> MSLSFCGNNISSYNIYHGVLQNPCFVDALNLVPHVFLLFITFPILFIGWGSQSSKVQIHHNTWLHFPGHNLRWILTFALLFVHVCEIAEGIVSDSQRASRHLHLFMPAVMGFVATTTSIVYYHNIETSNFPKLLLALFLYWVMAFITKTIKLVKYWQLGWGMSDLRFCITGVMVILNGLLMAVEINVIRVRRYVFFMNPQKVKPPEDLQDLGVRFLQPFVNLLSKATYWWMNTLIISAHRKPIDLKAIGKLPIAMRAVTNYVCLKEAYEEQKKKAADHPNRTPSIWLAMYRAFGRPILLSSTFRYLADLLGFAGPLCISGIVQRVNEPKNNTTRFSETLSSKEFLENAHVLAVLLFLALILQRTFLQASYYVTIETGINLRGALLAMIYNKILRLSTSNLSMGEMTLGQINNLVAIETNQLMWFLFLCPNLWAMPVQIIMGVILLYNLLGSSALVGAAVIVLLAPIQYFIATKLAEAQKSTLDYSTERLKKTNEILKGIKLLKLYAWEHIFCKSVEETRMKELSSLKTFALYTSLSIFMNAAIPIAAVLATFVTHAYASGNNLKPAEAFASLSLFHILVTPLFLLSTVVRFAVKAIISVQKLNEFLLSDEIGEDSWRTGEGTLPFESCKKHTGVQSKPINRKQPGRYHLDNYEQARRLRPAETEDVAIKVTNGYFSWGSGLATLSNIDIRIPTGQLTMIVGQVGCGKSSLLLAILGEMQTLEGKVYWNNVNESEPSFEATRSRSRYSVAYAAQKPWLLNATVEENITFGSSFNRQR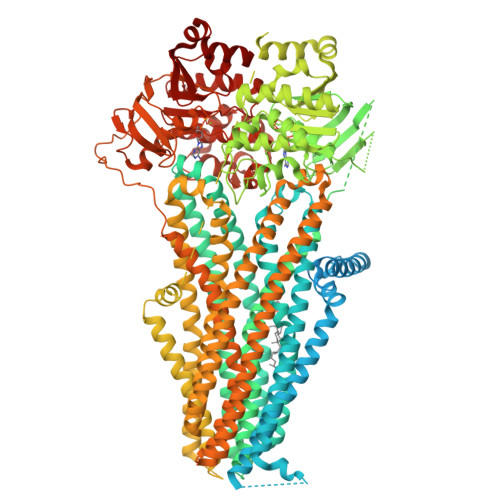YKAVTDACSLQPDIDLLPFGDQTEIGERGINLSGGQRQRICVARALYQNTNIVFLDDPFSALDIHLSDHLMQEGILKFLQDDKRTVVLVTHKLQYLTHADWIIAMKDGSVLREGTLKDIQTKDVELYEHWKTLMNRQDQELEKDMEADQTTLERKTLRRAMYSREAKAQMEDEDEEEEEEEDEDDNMSTVMRLRTKMPWKTCWWYLTSGGFFLLFLMIFSKLLKHSVIVAIDYWLATWTSEYSINDPGKADQTFYVAGFSILCGAGIFLCLVTSLTVEWMGLTAAKNLHHNLLNKIILGPIRFFDTTPLGLILNRFSADTNIIDQHIPPTLESLTRSTLLCLSAIGMISYATPVFLIALAPLGVAFYFIQKYFRVASKDLQELDDSTQLPLLCHFSETAEGLTTIRAFRHETRFKQRMLELTDTNNIAYLFLSAANRWLEVRTDYLGACIVLTASIASISGSSNSGLVGLGLLYALTITNYLNWVVRNLADLEVQMGAVKKVNSFLTMESENYEGTMDPSQVPEHWPQEGEIKIHDLCVRYENNLKPVLKHVKAYIKPGQKVGICGRTGSGKSSLSLAFFRMVDIFDGKIVIDGIDISKLPLHTLRSRLSIILQDPILFSGSIRFNLDPECKCTDDRLWEALEIAQLKNMVKSLPGGLDATVTEGGENFSVGQRQLFCLARAFVRKSSILIMDEATASIDMATENILQKVVMTAFADRTVVTIAHRVHTILTADLVIVMKRGNILEYDTPESLLAQEDGVFASFVRADM> SLPPVNTDIHDWVKTKGAWDKGYKGQGKVVAVIDTGIDPAHQSMRISDVSTAKVKSKEDMLARQKAAGINYGSWINDKVVFAHNYVENSDNIKENQFEDFDEDWENFEFDAEAEPKAIKKHKIYRPQSTQAPKETVIKTEETDGSHDIDWTQTDDDTKYESHGMHVTGIVAGNSKEAAATGERFLGIAPEAQVMFMRVFANDVMGSAESLFIKAIEDAVALGADVINLSLGTANGAQLSGSKPLMEAIEKAKKAGVSVVVAAGNERVYGSDHDDPLATNPDYGLVGSPSTGRTPTSVAAINSKWVIQRLMTVEELEKRADLNHGKAIYSESVDFKNIKDSLGYDKSHQFAYVKESTDAGYNAQDVKGKIALIERDPNKTYDEMIALAKKHGALGVLIFNNKPGQSNRSMRLTANGMGIPSAFISHEFGKAMSQLNGNGTGSLEFDSVVSKAPSQKGNEMNHFSNWGLTSDGYLKPDITAPGGDIYSTYNDNHYGSQTGTSMASPQIAGASLLVKQYLEKTQPNLPKEKIADIVKNLLMSNAQIHVNPETKTTTSPRQQGAGLLNIDGAVTSGLYVTGKDNYGSISLGNITDTMTFDVTVHNLSNKDKTLRYDTELLTDHVDPQKGRFTLTSRSLKTYQGGEVTVPANGKVTVRVTMDVSQFTKELTKQMPNGYYLEGFVRFRDSQDDQLNRVNIPFVGFKGQFENLAVAEESIYRLKSQGKTGFYFDESGPKDDIYVGKHFTGLVTLGSETNVSTKTISDNGLHTLGTFKNADGKFILEKNAQGNPVLAISPNGDNNQDFAAFKGVFLRKYQGLKASVYHASDKEHKNPLWVSPESFKGDKNFNSDIRFAKSTTLLGTAFSGKSLTGAELPDGYYHYVVSYYPDVVGAKRQEMTFDMILDRQKPVLSQATFDPETNRFKPEPLKDRGLAGVRKDSVFYLERKDNKPYTVTINDSYKYVSVEDNKTFVERQADGSFILPLDKAKLGDFYYMVEDFAGNVAIAKLGDHLPQTLGKTPIKLKLTDGNYQTKETLKDNLEMTQSDTGLVTNQAQLAVVHRNQPQSQLTKMNQDFFISPNEDGNKDFVAFKGLENNVYNDLTVNVYAKDDHQKQTPIWSSQAGAGASAIESTA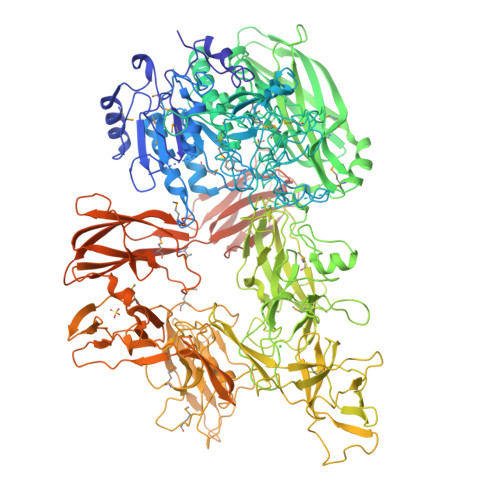WYGITARGSKVMPGDYQYVVTYRDEHGKEHQKQYTISVNDKKPMITQGRFDTINGVDHFTPDKTKALGSSGIVREEVFYLAKKNGRKFDVTEGKDGITVSDNKVYIPKNPDGSYTISKRDGVTLSDYYYLVEDRAGNVSFATLRDLKAVGKDKAVVNFGLDLPVPEDKQIVNFTYLVRDADGKPIENLEYYNNSGNSLILPYGKYTVELLTYDTNAAKLESDKIVSFTLSADNNFQQVTFKMTMLATSQITAHFDHLLPEGSRVSLKTAQGQLIPLEQSLYVPKAYGKTVQEGTYEVVVSLPKGYRIEGNTKVNTLPNEVHELSLRLVKVGDASDSTGDHKVMSKNNSQALTASATPTKTTTPATAKALPSTGEKMGLKLRIVGLVLLGLTCVFSRKKSTKD5'-azido-8-[(2-{[2-(1H-benzimidazol-2-yl)ethyl]amino}-2-oxoethyl)sulfanyl]-5'-deoxyadenosine 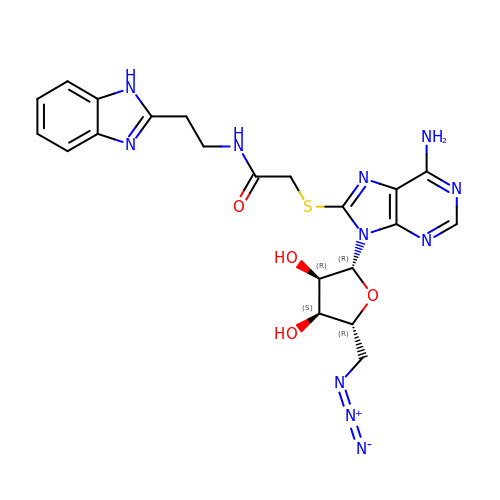| C21 H23 N11 O4 S | QNDDYPVSXWRDOZ-QQRWZLOUSA-N2-(4-AMINO-2-CHLOROPHENOXY)-5-CHLOROPHENOL | C12 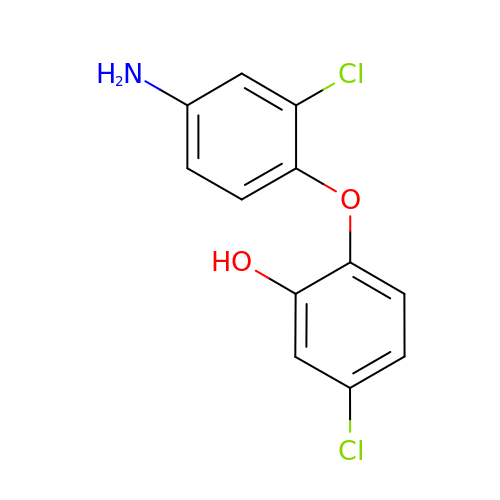H9 Cl2 N O2 | MCYCMAVHVQGDNE-UHFFFAOYSA-N[(1S,4r)-4-{4-[(4S)-2-({[4-(trifluoromethoxy)phenyl]methyl}carbamoyl)imidazo[1,2-a]pyridin-6-yl]phenyl}cyclohexyl]acetic acid | C30 H28 F3 N3 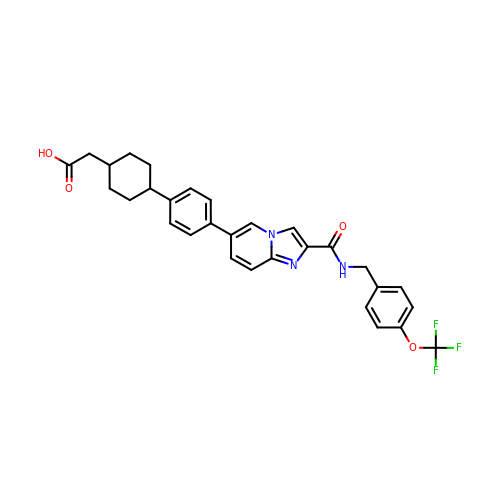O4 | KFGSQOIWOCDWAS-XUTJKUGGSA-N>AANEADYQAKLTAYQTELARVQKANADAKAAYEAAVAANNAANAALTAENTAIKKRNADAKADYEAKLAKYQADLAKYQKDLADYPVKLKAYEDEQTSIKAALAELEKHKNEDGNLTEPSAQNLVYDLEPNANLSLTTDGKFLKASAVDDAFSKSTSKAKYDQKILQLDDLDITNLEQSNDVASSMELYGNFGDKAGWSTTVSNNSQVKWGSVLLERGQSATATYTNLQNSYYNGKKISKIVYKYTVDPKSKFQGQKVWLGIFTDPTLGVFASAYTGQVEKNTSIFIKNEFTFY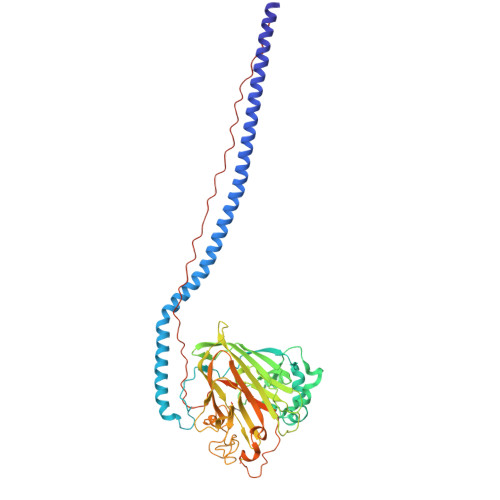DEDGKPINFDNALLSVASLNREHNSIEMAKDYSGKFVKISGSSIGEKNGMIYATDTLNFKQGEGGSRWTMYKNSQAGSGWDSSDAPNSWYGAGAIKMSGPNNYVTVGATSATNVMPVSDMPVVPGKDNTDGKKPNIWYSLNGKIRAVNVPKVTKEKPTPPVKPTAPTKPTYETEKPLKPAPVAPNYEKEPTPPTRLEHHHHHH[2x]>ANPCCSNPCQNRGECMSTGFDQYKCDCTRTGFYGENCTTPEFLTRIKLLLKPTPNTVHYILTHFKGVWNIVNNIPFLRSLIMKYVLTSRSYLIDSPPTYNVHYGYKSWEAFSNLSYYTRALPPVADDCPTPMGVKGNKELPDSKEVLEKVLLRREFIPDPQGSNMMFAFFAQHFTHQFFKTDHKRGPGFTRGLGHGVDLNHIYGETLDRQHKLRLFKDGKLKYQVIGGEVYPPTVKDTQVEMIYPPHIPENLQFAVGQEVFGLVPGLMMYATIWLREHNRVCDILKQEHPEWGDEQLFQTSRLILIGETIKIVIEDYVQHLSGYHFKLKFDPELLFNQQFQYQNRIASEFNTLYHWHPLLPDTFNIEDQ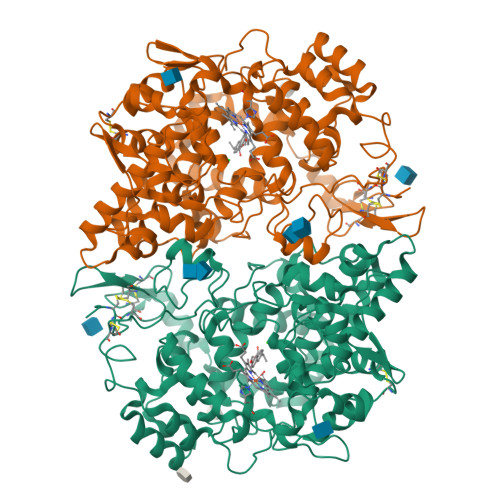EYSFKQFLYNNSILLEHGLTQFVESFTRQIAGRVAGGRNVPIAVQAVAKASIDQSREMKYQSLNEYRKRFSLKPYTSFEELTGEKEMAAELKALYSDIDVMELYPALLVEKPRPDAIFGETMVELGAPFSLKGLMGNPICSPQYWKPSTFGGEVGFKIINTASIQSLICNNVKGCPFTSFNVQDPQPTKTATINASASHSRLDDINPTVLIKRRSTEL[2x]>[2x]MHHHHHHNEEFRPEMLQGKKVIVTGASKGIGREMAYHLSKMGAHVVLTARSEEGLQKVVSRCLELGAASAHYIAGTM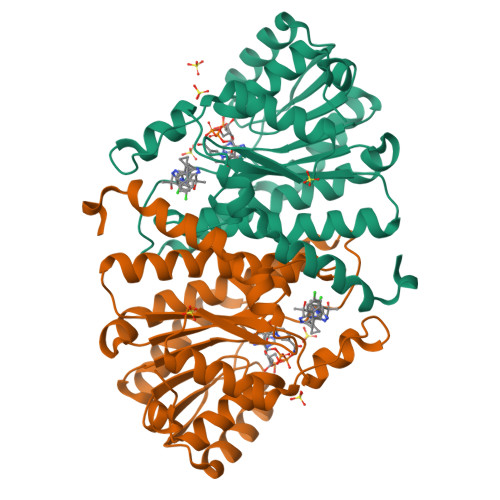EDMTFAEQFIVKAGKLMGGLDMLILNHITQTSLSLFHDDIHSVRRVMEVNFLSYVVMSTAALPMLKQSNGSIAVISSLAGKMTQPMIAPYSASKFALDGFFSTIRTELYITKVNVSITLCVLGLIDTETAMKEISGIINAQASPKEECALEIIKGTALRKSEVYYDKSPLTPILLGNPGRKIMEFFSLRYYNKDMFVSN> EALSSKVQQLERSIGLKDLAMADLEQKVLEMEASTYD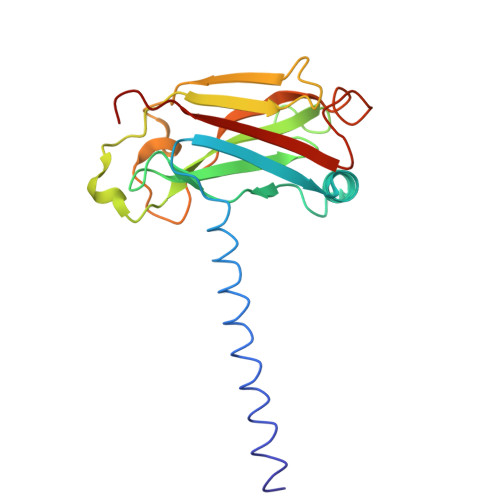GVFIWKISDFPRKRQEAVAGRIPAIFSPAFYTSRYGYKMCLRIYLNGDGTGRGTHLSLFFVVMKGPNDALLRWPFNQKVTLMLLDQNNREHVIDAFRPDVTSSSFQRPVNDMNIASGCPLFCPVSKMEAKNSYVRDDAIFIKAIVDLTGL>GPLGS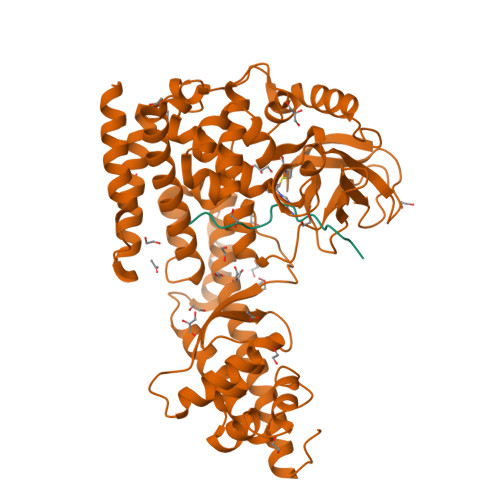MGKKSRVKTQKSGTGATATVSPKEILNLTSELLQKCSSPAPGPGKEWEEYVQIRTLVEKIRKKQKGLSVTFDGKREDYFPDLMKWASENGASVEGFEMVNFKEEGFGLRATRDIKAEELFLWVPRKLLMTVESAKNSVLGPLYSQDRILQAMGNIALAFHLLCERASPNSFWQPYIQTLPSEYDTPLYFEEDEVRYLQSTQAIHDVFSQYKNTARQYAYFYKVIQTHPHANKLPLKDSFTYEDYRWAVSSVMTRQNQIPTEDGSRVTLALIPLWDMCNHTNGLITTGYNLEDDRCECVALQDFRAGEQIYIFYGTRSNAEFVIHSGFFFDNNSHDRVKIKLGVSKSDRLYAMKAEVLARAGIPTSSVFALHFTEPPISAQLLAFLRVFCMTEEELKEHLLGDSAIDRIFTLGNSEFPVSWDNEVKLWTFLEDRASLLLKTYKTTIEEDKSVLKNHDLSVRAKMAIKLRLGEKEILEKAVKSAAVNREYYRQQMEEKAPLPKYEESNLGLLESSVGDSRLPLVLRNLEEEAGVQDALNIREAISKAKATENGLVNGENSIPNGTRSENESLNQESKRAVEDAKGSSSDSTAGVKE[2x];>[2x]TLKYPIEHGIVTNWD L-RhI is one of the enzymes involved in L-rhamnose metabolism and catalyzes the reversible isomerization between L-rhamnose and L-rhamnulose. Herein, we report the crystal structures of L. rhamnosus Probio-M9 L-RhI (LrL-RhI) in complexes with L-rhamnose, D-allulose, and D-allose, which show enzyme activity toward L-rhamnose, D-allulose, and D-allose in acidic conditions, though the activity toward D-allose was low. All structures belong to the orthorhombic space group P212121 with four molecules (Mol-A, Mol-B, Mol-C, and Mol-D) forming a homotetramer in an asymmetric unit. The overall structure of LrL-RhI is similar to the known structures of L-RhIs.

Four crystal structures, such as LrL-RhI alone and complexes with L-rhamnose (LrL-RhI/L-rhamnose), D-allulose (LrL-RhI/D-allulose), and D-allose (LrL-RhI/D-allose), were determined at resolutions of 1.90, 1.61, 1.73, and 1.71 Å, respectively. The structural metal (Mn1) is coordinated by Glu228, Asp261, His288, and Asp328, and the catalytic metal (Mn2) is coordinated by His264, Asp296, Asp298, and three water molecules (W4, W5, and W6). The bound metal ions with strong electron density maps were refined as Mn2+ since LrL-RhI was expressed in cells in a medium containing 1 mM MnCl2. A part of the flexible loop region (Asp46-Thr73) was almost missing in the structures of LrL-RhI alone (missing Asn54-Ser64) and complexes with L-rhamnose (missing Pro53-Ser64) and D-allose (missing Asn54-Gly65) due to the weak electron density maps, but the corresponding region in the structure of LrL-RhI/D-allulose (Mol-A and Mol-B) was relatively visible, and a part of the region (Asn54-Gly65) was refined with 50% occupancy.

>[4x]MVKPEEVDKAYEVAKQRYAEIGVDTDAAMKELEKVPLSVHCWQGDDIHGFLFPNQELTGGIGVSGNYPGIARTPDELAGDMHEALSLIPGKHRVQLHAIYAVTDKKRDLDTLEPEDFDYWIDWAKQEGVGLDFNGTFFSHPMVKDNMTVSSPDPKVRDFWIRHGKISREISNYIGEKLGSQVVNNFWLPDGFKDNPIDKKTPRLRLLKALDEIIKDPLPEKNTIESFEGKLFGTGIESYTTGSHEFYQNYAISRNKLWTIDAGHFHPTEDVSDKFSAFFPFGKGLFMHVSRPVRWDSDHVVIMDDALIRITRSLVRDGYLDRTHIGLDFFDATINRVAAWVVGARATQKSLLQAMLAPIDQLKKDELNADFTTRLIETEELKSFPFGAVWDKFCQDHNTPVGFDWMNNIHQYEKDVQFKRDAKLVHGSHHHHHH> MTIFNLYIFDKFGTLLHYAEWNRTKKSGITRE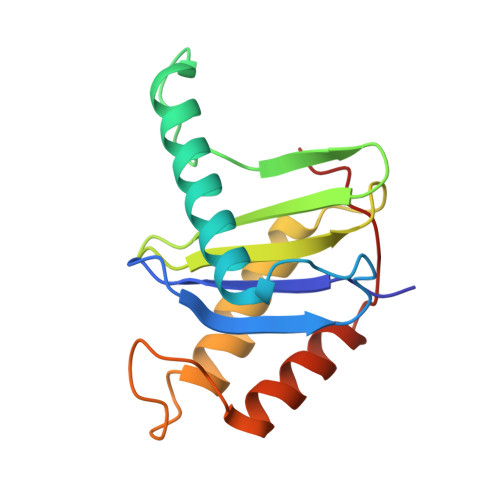EEAKLTYGMLFSIKSFVSKISPHDPKEGFLYYKTNRYALHYLETPSGLKFVLNTDTTAINVKELLQQLYAKVWVEFVVRDPLWTPGTVVTSELFQSKLDEFVRQSPIFGIRNI> QDPRNSGSDCLLSKEQLRSIYESSLSIGNFASRLLVHL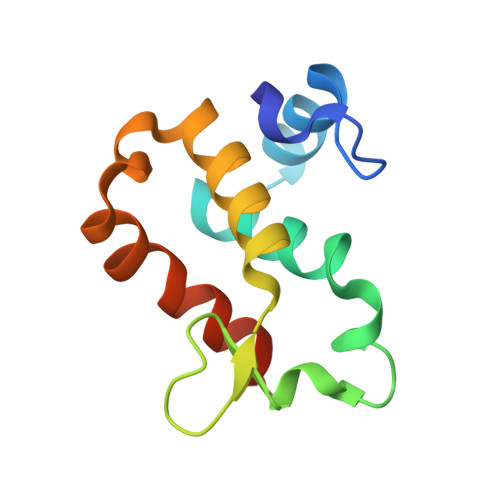FPELFTHENLRKQYNCSGSLGKKQLDPARIRLIRHYVQLLYPRAKNDRVWTLEFVGKLDERCRRRDTEQ>[4x]IIGGRESRPHSRPYMAYLQIQSPAGQSRCGGFLVREDFVLTAAHCWGSNINVTLGAHNIQRRENTQQHITARRAIRHPQYNQRTIQNDIMLLQLSRRVRRNRNVNPVALPRAQEGLRPGTLCTVAGWGRVSMRRGTDTLREVQLRVQRDRQCLRIFGSYDPRRQICVGDRRERKAAFKGDSG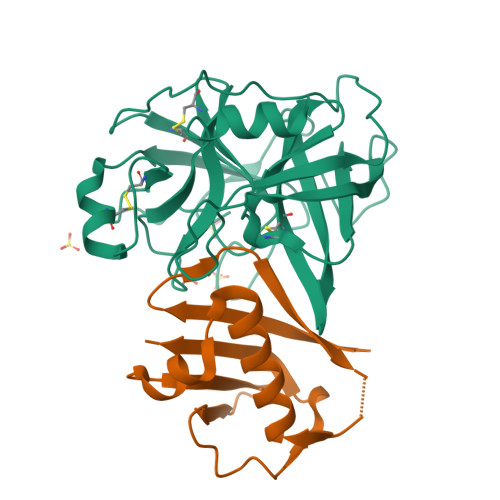GPLLCNNVAHGIVSYGKSSGVPPEVFTRVSSFLPWIRTTMRS;>[4x]GKHTVPYTISVDGITALHRTYFVFPENKKVLYQEIDSKVKNELASQRGVTTEKINNAQTATYTLTLNDGNKKVVNLKKNDDAKNSIDPSTIKQIQIVVK>[2x]QTSSGRNFFRKKVMGNRRSDEPAKTKKGLSSILDAARWNRGEPQVPDFRHLKAEVDAEKPGATDRKGGVGMPSRDRNIGAPGQDTPGVSLHPLSLDSPDREPGADAPLELGDSSPQGPMSLESLAPPESTDEGAETESPEPGDEGEPGRSGLELEPEEPPGWRELVPPDTLHSLPKSQVKRQEVISELLVTEAAHVRMLRVLHDLFFQPMAECLFFPLEELQNIFPSLDELIEVHSLFLDRLMKRRQESGYLIEEIGDVLLARFDGAEGSWFQKISSRFCSRQSFALEQLKAKQRKDPRFCAFVQEAESRPRCRRLQLKDMIPTEMQRLTKYPLLLQSIGQNTEEPTEREKVELAAECCREIL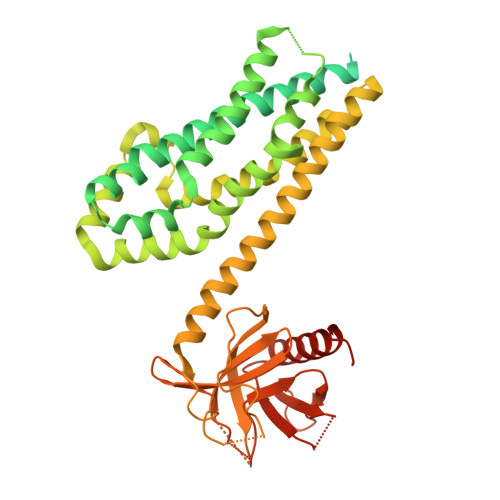HHVNQAVRDMEDLLRLKDYQRRLDLSHLRQSSDPMLSEFKNLDITKKKLVHEGPLTWRVTKDKAVEVHVLLLDDLLLLLQRQDERLLLKSHSRTLTPTPDGKTMLRPVLRLTSAMTREVATDHKAFYVLFTWDQEAQIYELVAQTVSERKNWCALITETAGSLKVPAHHHHHH> MSLVKMRDKILGSVFGAVIGDALGMPTENLTKEEIKKLYGFVDSYVEPKNYLAGKLNKGEWTDDTEQAICLIKSLTKEGIDIKKFANCLIAWKNKNPPDIGLTSLMAIDKLENNDYSGVDSSSCGAAMRIYPLGIVFHNNLKKLKEEVIKASKITHNNKTAIAGALAIAFFVSSALKDRKDFSLLDECYNYIKDIDEEFAKKLLEI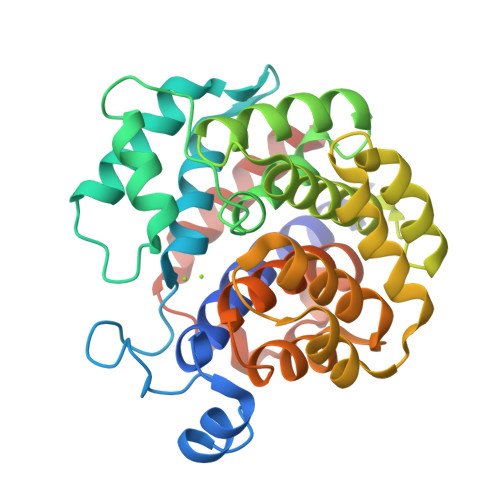KNFNNLDYIYDYFGTGVKTDEVVPSAIATYLLTDNFKEGMLKCINAGGDTDSLASMYGAMAGAYYGFKNIPKEWIDGLKNKEVIFELAERLYHLATEEGGSHHHHHH>TQQFSILPGNKAFKGKFTVPGDKSVSHRSIMFGAIAEGTTHVTGFLEGEDALATLQAFRDMGVSIEGPKNGEVTIHGVGMHGLKAPASALYMGNSGTSMRLLSGMLSAQKFDSVMTGDASLSKRPMERIAKPLRLMGAQIQTTGEKGTPPVSITGGQQLKGIQYDLPMASAQVKSGILLAGLWAEGETSVTEPEPTRDHTERMLRAFGYDVKTEGNKISLVGGGKLVGTNIQVPSDISSAAFFMVGAAITEGADVVLEAVGINPTRTGVIE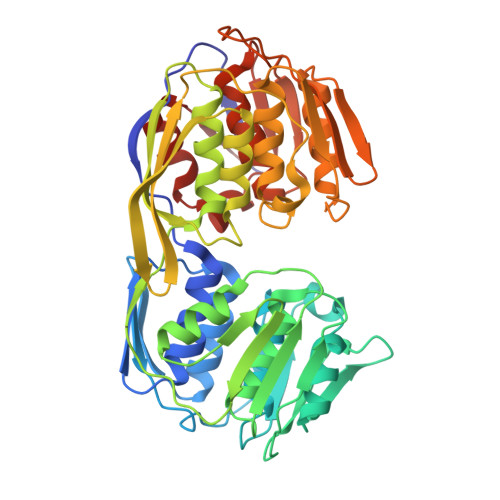ILKQMGADLTVENERIAGGEPIADIHIKGSRTLKGIHMPEDQVPLAIDEFPALFIAAACAEGQTVLTGAAELRVKESDRIQVMADGLKIMGIDCTPTEDGIIIEGKGKSGDWSPIFAGGEIESHHDHRIAMSFSMAGLRTSGPITIHGTETVATSFPTFTELANRAGLTIEVSQ[2x]> GANAMDEITVVLKSPNGKNIKCPPMPRKDFSRAEVLGYIGMCSGAQRFEIASLKTPKFGENLLKIIKSKGSQSFIVDCTDEEIDQFSAETKSGSNA

Type III CRISPR systems detect invading RNA and activate the catalytic Cas10 subunit, which generates a range of nucleotide second messengers to signal infection. Csx23 provides immunity against plasmids and phage when expressed in Escherichia coli along with its cognate type III CRISPR system. The Csx23 protein localises in the membrane using an N-terminal transmembrane α-helical domain and has a cytoplasmic C-terminal domain that binds cyclic tetra-adenylate (cA4), activating its defence function. Csx23 is activated by cA4 to prevent successful phage infection, most likely by disruption of the host membrane integrity.

To investigate cA4 binding by Csx23 at an atomic level, we co-crystallised the soluble CTD of Csx23 with cA4. Diffraction data were collected on the crystals to a resolution of 1.76 Å, and the structure was solved using molecular replacement with the monomeric AF2 model as the search model. The asymmetric unit contains one protomer of Csx23 CTD, comprising two beta-strands, linked via two alpha-helices to a third beta-strand, which together form a mixed anti-parallel/parallel beta-sheet, followed by a short alpha-helix at the C-terminus. Interestingly, the 4-fold crystallographic symmetry creates a tetrameric arrangement of Csx23 CTD, which is consistent with the behaviour of the protein in the presence of cA4 observed by cross-linking. The cA4 molecule, and a coordinating sodium ion, are positioned at the centre of rotation for the 4-fold crystallographic symmetry, meaning there is effectively one adenylate moiety bound to one Csx23 CTD protomer in the asymmetric unit; cA4 and the sodium ion were modelled with 0.25 occupancy to account for this. R95 of Csx23 CTD makes electrostatic interactions between both terminal nitrogen atoms and two different oxygen atoms in the phosphate group of cA4. R110 and F111 sandwich the adenine base in cA4 through π–π interactions. Whilst R95 is positioned deep into the cA4 binding cavity, both R110 and F111 are located on a loop (comprising residues 107–113) on the surface of the Csx23 CTD. This loop must display flexibility to allow cA4 access to the binding cavity, and then changes conformation to close over cA4 once bound. The structural fold observed for Csx23 CTD is novel compared to other structures reported to bind cA4 (and other cOAs), demonstrating both the structural and functional diversity in the proteins that have evolved to interact with cyclic nucleotides.>MTASTLPRSDVEFTTLDGLTLRGWLFPAS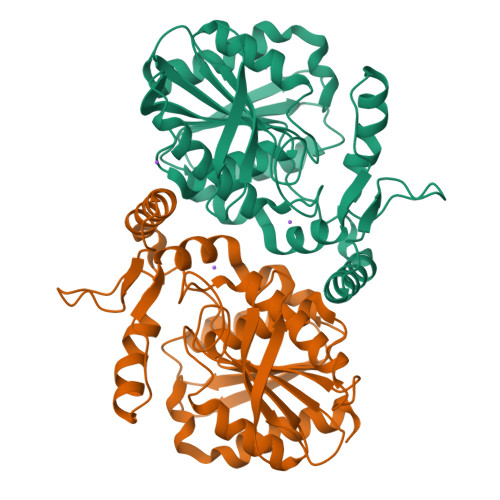QRGPALIMSPGFNMPKDAILPDIAKWFQEHGITCLLYDPRGIGASDGEPRNDIDARQQAEHLHDAVTWFKENPLVNEKQIALWGLCFGGNVTLAAAAFDKRVAAAIAVAPLIDSTGNPERRQPILELAMHDRASRLDGEEPMYLPYVNEDGSIPNGLQLAAEMMPALERLGIPVENRISVQTYYKSLSWNILNVVQYISPTPAMMVTPELDVSCPTEDQLNCFEHMKEPKELDILKGKGHLDWVFGDVESILNRQLDFLKRHMAF[2x]The PsbQ-like protein, termed CyanoQ, found in the cyanobacterium Synechocystis sp. PCC 6803 is thought to bind to the lumenal surface of photosystem II (PSII), helping to shield the Mn4CaO5 oxygen-evolving cluster. Here, we show that CyanoQ (encoded by tll2057) is indeed expressed in the thermophilic cyanobacterium Thermosynechococcus elongatus and provide evidence in support of its assignment as a lipoprotein. Using an immunochemical approach, we show that CyanoQ co-purifies with PSII and is actually present in highly pure PSII samples used to generate PSII crystals. We have also determined the crystal structure of CyanoQ from T. elongatus to a resolution of 1.6 Å.

To gain insights into the structure of CyanoQ from T. elongatus, a cleavable N-terminal His6-tagged derivative lacking the predicted lipidated Cys24 residue was over-expressed in E. coli and the protein purified by immobilised nickel-affinity chromatography to near homogeneity. The predicted product contains residues 25–152 of CyanoQ plus 5 additional residues (GSELE) at the N-terminus. The first nine N-terminal residues as well as the last C-terminal residue of CyanoQ could not be detected in the electron density map so only residues 34–151 were fitted. Topologically the protein belongs to four-helix bundle superfamily and its fold is classified as mainly alpha up-down bundle (CATH 1.20.120.290) with four α-helices, of which the first two are broken, and one 310 helix. The first amino-acid residue of helix 2a, Trp71, is absolutely conserved in the analysed CyanoQ sequences. The indole nitrogen is exposed towards the solvent, and in this structure a 2.8 Å hydrogen bond is created between Trp71Nε1 and Asp125Oδ1. The other absolutely conserved residues are found right after the C-terminus of helix 2a and consist of a Gly80Pro81 motif that is immediately preceded by a positively charged amino acid, either arginine as in T. elongatus or in most cases histidine. Both glycine and proline are well known as the most efficient ‘helix breakers’ and in fact they separate helix 2a from helix 2b in CyanoQ. In the case of T. elongatus the larger H2-H3 cavity is composed of a cluster of Met78, Arg79, Leu82, Phe115 and Asp119 surrounding the Gly80Pro81 motif. Despite the fact that five out of the six corresponding positions are occupied by potential metal ligands in T. elongatus CyanoQ, no zinc cations are present in the crystal structure. Although there were no bound Zn2+ ions in our structure, we were able to fit a sulphate ion into the electron density.

> GSGGPSATTPPPPTYSELQITRIQDYLRDIEKNAERFADLEVSVAKGDWQEARNIMRGPLGEMLMDMRALNRNLLAKDQPTPTALTRALTDDFLKIDQGADLDSVTVAQEGFREAEADFKAYLNSLPELS> YVEFEPSDKHIKEYLNKIQNSLSTEWSPCSVTCGNGIQVRIKPGSANKPKDELDYANDIEK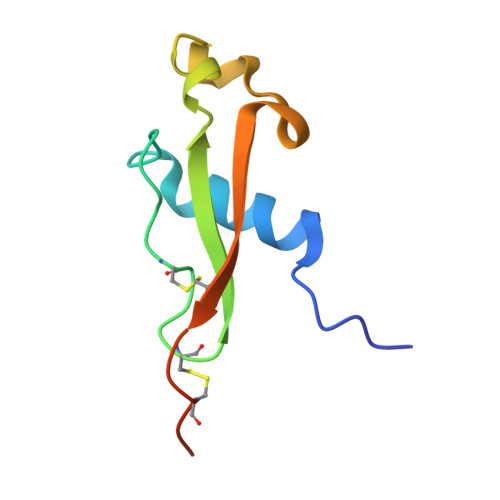KICKMEKCPHHHHHHA> IVGGYTCGANTVPYQVSLNSGYHFCGGSLINSQWVVSAAHCYKSGIQVRLGEDNINVVEGNEQFISASKSIVHPSYNSNTLNNDIMLIKLKSAASLNSRVASISLPTSCASAGTQCLISGWGNTKSSGTSYPDVLKCLKAPILSDSSCKSASSYIITSN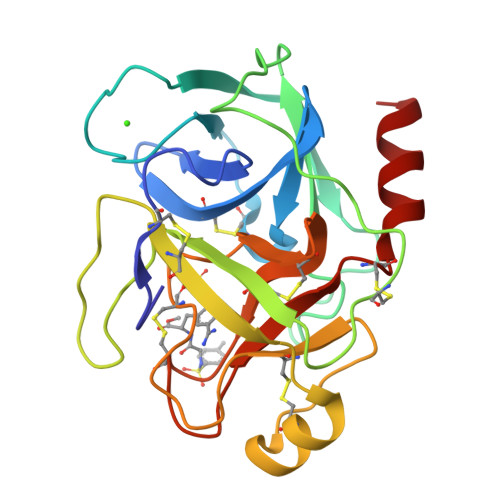MFCAGYLEGGKDSCQGDSGGPVVCSGKLQGIVSWGSGCAQKNKPGVYTKVCNYVSWIKQTIASN> NTKGIDEIKNLETDFNGRIGVYALDTGSGK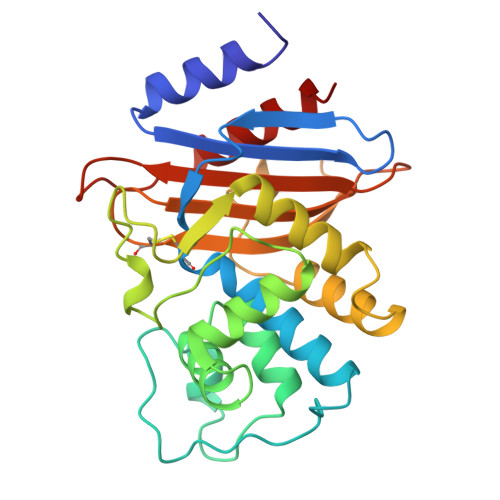SFSYRANERFPLCSSFKGFLAAAVLKGSQDNRLNLNQIVNYNTRSLEFHSPITTKYKDNGMSLGDMAAAALQYSDNGATNIILERYIGGPEGMTKFMRSIGDEDFRLDRWELDLNTAIPGDERDTSTPAAVAKSLKTLALGNILSEHEKETYQTWLKGNTTGAARIRASVPSDWVVGDKTGSCGAYGTANDYAVVWPKNRAPLIISVYTTKNEKEAKHEDKVIAEASRIAIDNLK>[2x]MAHAMENSWTISKEYHIDEEVGFALPNPQENLPDFYNDWMFIAKHLPDLIESGQLRERVEKLNMLSIDHLTDHKSQRLARLVLGCITMAYVWGKGHGDVRKVLPRNIAVPYCQLSKKLELPPILVYADCVLANWKKKDPNKPLTYENMDVLFSFRDGDCSKGFFLVSLLVEIAAASAIKVIPTVFKAMQMQERDTLLKALLEIASCLEKALQVFHQIHDHVNPKAFFSVLRIYLS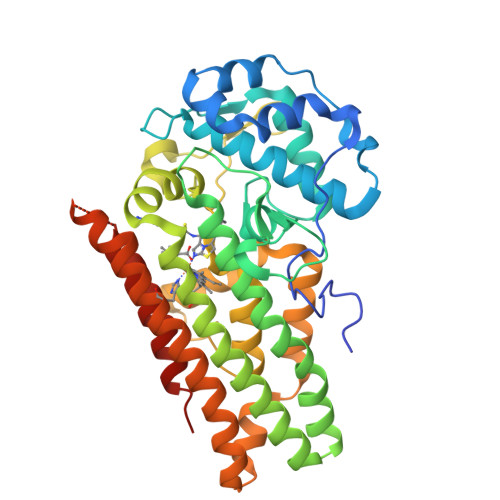GWKGNPQLSDGLVYEGFWEDPKEFAGGSAGQSSVFQCFDVLLGIQQTAGGGHAAQFLQDMRRYMPPAHRNFLCSLESNPSVREFVLSKGDAGLREAYDACVKALVSLRSYHLQIVTKYILIPASQQPKENKTSEDPSKLEAKGTGGTDLMNFLKTVRSTTEKSLLKEG>[4x]SMAMFYAHALGGYDENLHAFPGISSTVANDVRKYSVVSVYNNK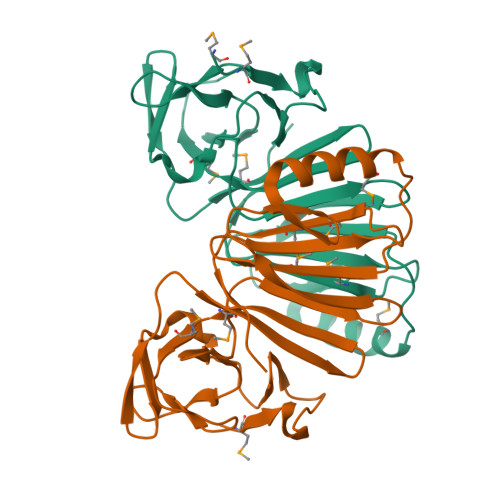YDIVKDKYMWCYSQVNKRYIGALLPMFECNEYLQIGDPIHDQEGNQISIITYRHKNYYALSGIGYESLDLCLEGVGIHHHVLETGNAVYGKVQHDYSTIKEKAKEMNALSPGPIIDYHVWIGDCICQVTAVDVHGKEIMRMRFKKGAVLPIPNLVKVKLGENDTENLSSTISAAPSR5-[(3~{a}~{S},4~{S},6~{a}~{R})-2-oxidanylidene-1,3,3~{a},4,6,6~{a}-hexahydrothieno[3,4-d]imidazol-4-yl]-~{N}-[4-(2-azanylethylsulfamoyl)phenyl]pentanamide | C18 H27 N5 O4 S2 | 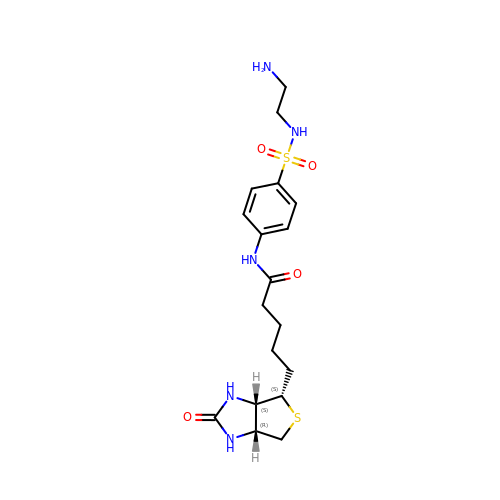ZDLCBMIPYXADBN-ZOBUZTSGSA-N> MASTTRLVNDRKQLEQQVKDDARILADARGLNITTVANDSATGGQAIRNVGPNDEATIKALDNVIKQIEALSVIVNRSEKADDAQILGPNTYKQLLEHLFSPEENVYILLPIQAYTGGVIDRRDASFSNFAYSIASKLMMELSAATHNKIFTDYTRIAASALGPEISTEGMPLFSLIESLELTEAETSRLPVIQDSMVIQKSTATVGNAQQGISTINIKRVPFVGSAFQQVIDQLLWEYSTTSLTTKEQRRQRITEMVNDRRIMIQKLTLAEKPQVMRHVTTEINNDLFFKMSPVAQLYI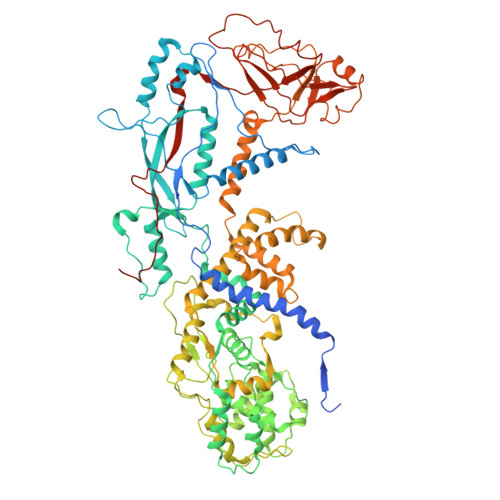YHLDRAFLDGVGFTPLAEKQQQLQLQLKTNILTANLIRSAINGMNTESNLEVAIKMMQAAQLHRASIEIAFPMNVSLSPEIIVQCFIVWMSIPEQLLSDRSNFIIAAVIWAGFSADDSYADIMRRSARASDRQNYDIIKAALSSRKFKLPRASTTLFDENEPVVRRYQIGRVYAPFPVDRYGSPVYSNCTKVELASDYNAEGFTIRKDDFRALQAVLRIDEDRAADMFTTLRIMISSIPAVWYDAEVVHYPHTAVELEQLAAYGLTGAYPRTNHSVDTIVKTVNNISATYSTIAQMLSTIDLDPTRYGTSESIDKFKIAWENVESVLNMEGNDFVKTIMYAYEDNFPKKDFYMMLKQIASDGQGAHPIAAAIDQLRTIVYREPERFGYIDSVILTHNPDVDTAYNRFFHLHPIVTNQPSNTIKNAQLWNEMRLEQQVEHIKAGPVRIIGPFHVTYNYLSEEEDMPATSHIIMKDNMILNDHLTFNFVKRERRNNKKRVSSFRYKAVEMYVAVRISRFQLEVLRDLHDLVRSRTYLDVSKSPLATTPIRVVEYVR>[2x]GPLGSHFHVFVGDLSPEITTAAIA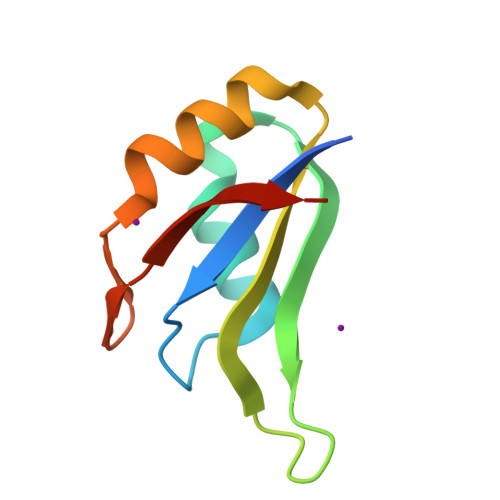AAFAPFGRISDARVVKDMATGKSKGYGFVSFFNKWDAENAIQQMGGQWLGGRQIRTNWATRKP> MDDLKLPRQRVDLVAPPFVHVHEQATKQGPKIMEFKLVVQEKKMVIDEKGTTFQAMTFNGSMPGPLMVVHEGDYVEVTLVNPATNTMPHNIDFHSATGALGGGALTLINPGEQVV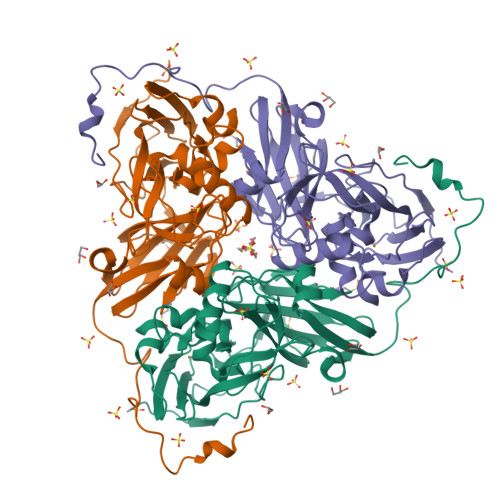LRWKATRTGVFVYHCAPGGPMIPWHVVSGMNGAVMVLPRDGLNDGHGHSLRYDRIYYIGEQDLYVPRDEKGNFKSYDSPGEAYSDTEEVMRKLTPTHVVFNGKAGALTGKNALNANVGENVLIVHSQANRDSRPHLIGGHGDYVWETGKFSNAPETGLETWFIRGGSAGAALYKFLQPGIYAYVTHNLIEAANLGATAHFKVEGKWNDDLMTQVKAPADIPTGSTNENLYFQ2-{4-[(2,5-difluorophenyl)methoxy]phenoxy}-5-ethoxyaniline 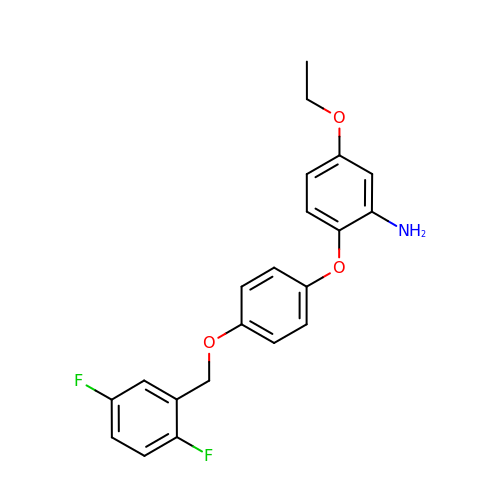| C21 H19 F2 N O3 | YSUBLPUJDOWYDP-UHFFFAOYSA-N> GSSHHHHHHS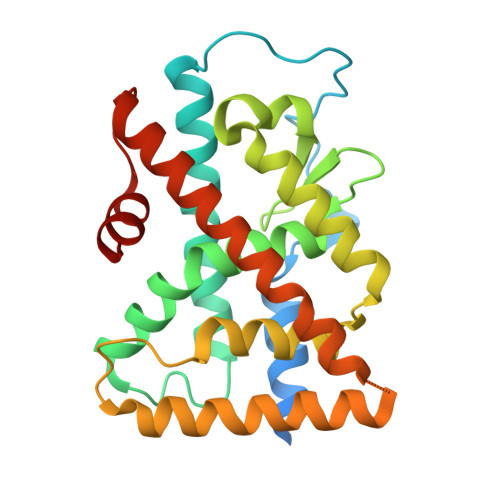SGLVPRGSHMQPPDASPTNLLTSLIRAHLDSGPNTAKLDYSKFQELVLPRFGKEDAGDVQQFYDLLSGSLDVIRKWAEKIPGFIELSPGDQDLLLESAFLELFILRLAYRSKPGEGKLIFCSGLVLHRLQCARGFGDWIDNILAFSRSLHSLGVDVPAFACLSALVLITDRHGLQDPRRVEELQNRIASCLKEHMAAVAGDPQPASCLSRLLGKLPELRTLCTQGLQRIFCLKLEDLVPPPPIVDKIFMDTLSF> GPDSMSANNGVTGKLSSRVMNMKFMKFGKTDDEESSNSNTPSNINSDVEPIEQKGKLFGLDDSAWDLNSYKDDLKKISGKEKKKVKRVVYKKRPNLIISNVGYSELRKPEGVISGRKTFGDNSDDSGSRKRKFDEGE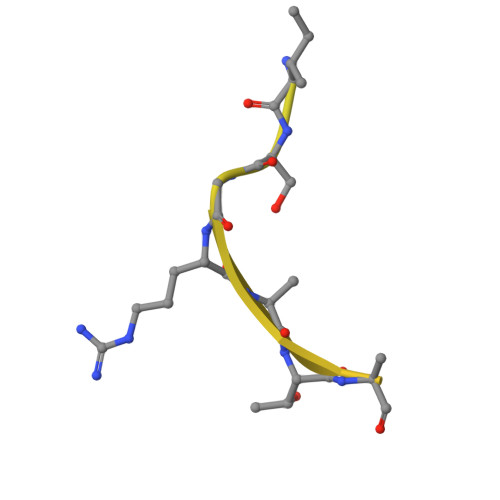QNEDEKRDAKDKEFTGSQDDGEDEYDLDKLFKDSIKKKKTNHNGKNKNRNSKK> RRRRR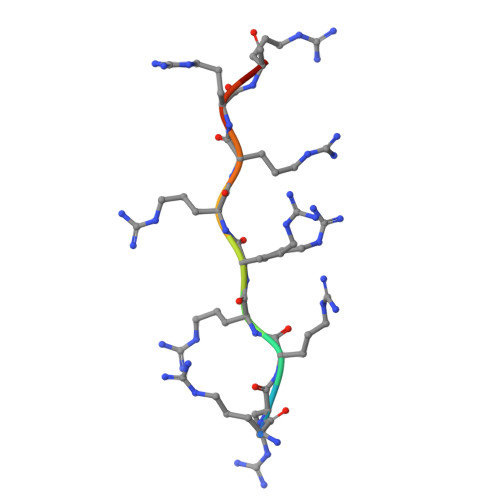RRRRR> MASERLPNRPACLLVASGAAEGVSAQSFLHCFTMASTAFNLQVATPGGKAMEFVDVTESNARWVQDFR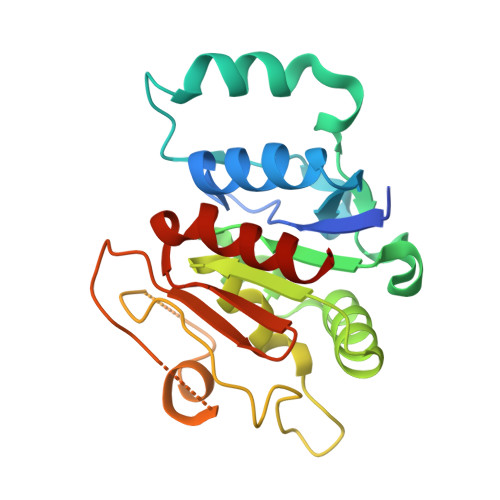LKAYASPAKLESIDGARYHALLIPSCPGALTDLASSGSLARILQHFHSESKPICAVGHGVAALCCATNEDRSWVFDSYSLTGPSVCELVRAPGFARLPLVVEDFVKDSGACFSASEPDAVHVVLDRHLVTGQNASSTVPAVQNLLFLCGSRK>[2x]TRDQNGTWEMESNENFEGY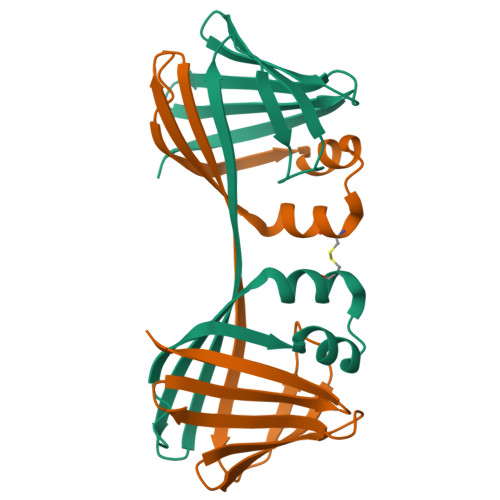MKALDIDFCTRKIAVRCTQTKVIDQDGDNFKDKTTSTFHRNYDVDFTVGVEFDEYTKSLDNRHVKALVTWEGDVLVCVQKGEKENRGWKKWIEGDKLYLELTCGDQVCRQVFKKK{(2S)-7-nitro-2-[(propan-2-ylamino)methyl]-1,2,3,4-tetrahydroquinolin-6-yl}methanol | C14 H21 N3 O3 | 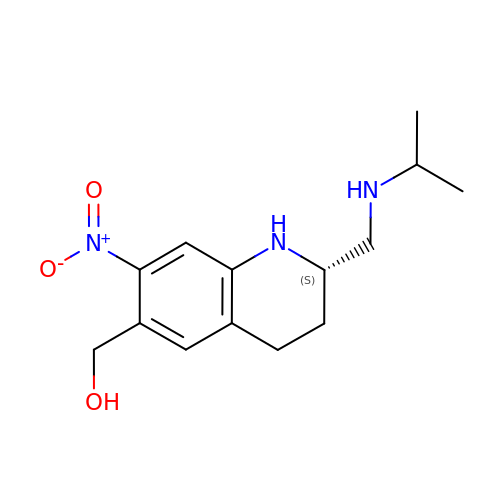XCGYUJZMCCFSRP-LBPRGKRZSA-N>QDSTSDLIPAPPLSKVPLQQNFQDNQFHGKWYVVGRAGNTGLREDKDPGKMFATIYELKEDKSYNVTYVWFGQKKCMYSIGTFVPGSQPGEFTLGNIKSAPGRTSWLVRVVSTNYNQHAMVFFKSVTQNREGFAITLYGRTKELTSELKENFIRFSKSLGLPENHIVFPVPIDQCIDGSAHHHHHH[2x];>[2x]ASWSHPQFEKGAELPAQKWWHTGALYRIGDLQAFQGHGAGNLAGLKGRLDYLSSLKVKGLVLGPIHKNQKDDVAQTDLLQIDPNFGSKEDFDSLLQSAKKKSIRVILDLTPNYRGENSWFSTQVDTVATKVKDALEFWLQAGVDGFQVRDIENLKDASSFLAEWQNITKGFSEDRLLIAGTNSSDLQQILSLLESNKDLLLTSSYLSDSGSTGEHTKSLVTQYLNATGNRWCSWSLSQARLLTSFLPAQLLRLYQLMLFTLPGTPVFSYGDEIGLDAAALPGQPMEAPVMLWDESSFPDIPGAVSANMTVKGQSEDPGSLLSLFRRLSDQRSKERSLLHGDFHAFSAGPGLFSYIRHWDQNERFLVVLNFGDVGLSAGLQASDLPASASLPAKADLLLSTQPGREEGSP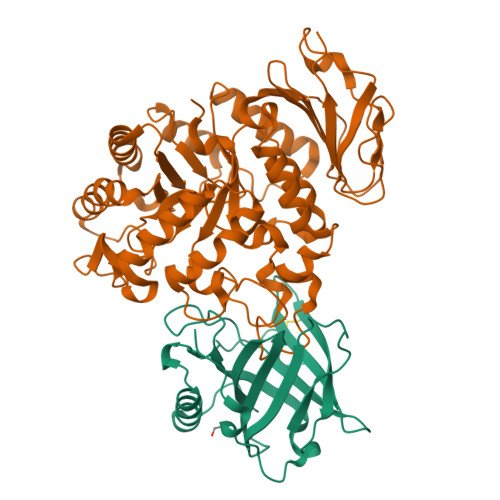LELERLKLEPHEGLLLRFPYAA>[2x]GSHMDTSLAEEVQQTMATLAPNRFFFMSPYRSFTTSGCF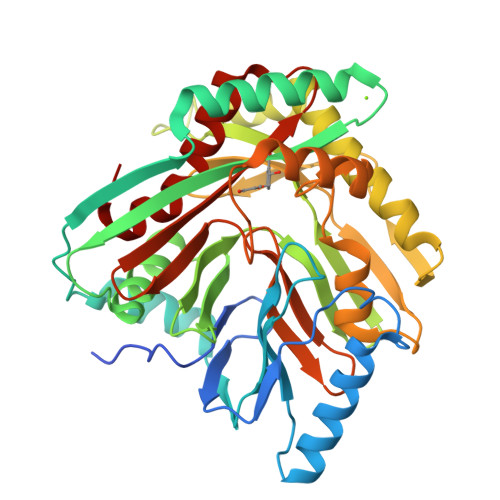ARFDEPAVNGDSPDSPFQQKLAALFADAKAQGIKNPVMVGAIPFDPRQPSSLYIPESWQSFSRQEKQASARRFTRSQSLNVVERQAIPEQTTFEQMVARAAALTATPQVDKVVLSRLIDITTDAAIDSGVLLERLIAQNPVSYNFHVPLADGGVLLGASPELLLRKDGERFSSIPLAGSARRQPDEVLDREAGNRLLASEKDRHEHELVTQAMKEVLRERSSELHVPSSPQLITTPTLWHLATPFEGKANSQENALTLACLLHPTPALSGFPHQAATQVIAELEPFDRELFGGIVGWCDSEGNGEWVVTIRCAKLRENQVRLFAGAGIVPASSPLGEWRETGVKLSTMLNVFGLH> GSDYIIKEKTVLLQKKDSEGFGFVLRGAKAQTPIEEFTPTPAFPALQYLESVDEGGVAWRAGLRMGDFLIEVNGQNVVKVGHRQVVNMIRQGGNTLMVKVVMVTRHPD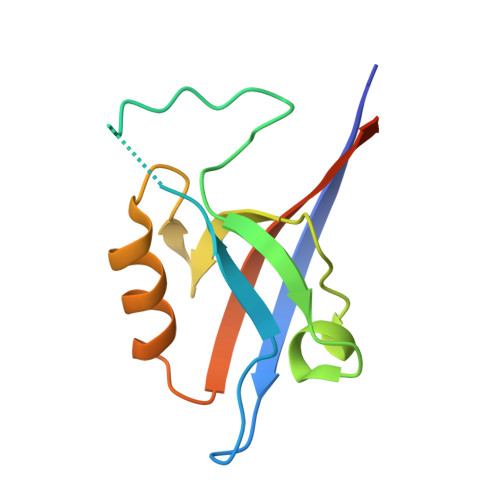MDEAVHK>[2x]QTLLDALNVRVVGSGERVLVLAHGFGTDQSAWNRILPFFLRDYRVVLYDLVCAGSVNPDFFDFRRYTTLDPYVDDLLHILDALGIDQCAYVGHSVSAMIGILASIRRPELFSKLILIGASPRFLNDEDYHGGFEQGEIEKVFSAMEANYEAWVNGFAPLA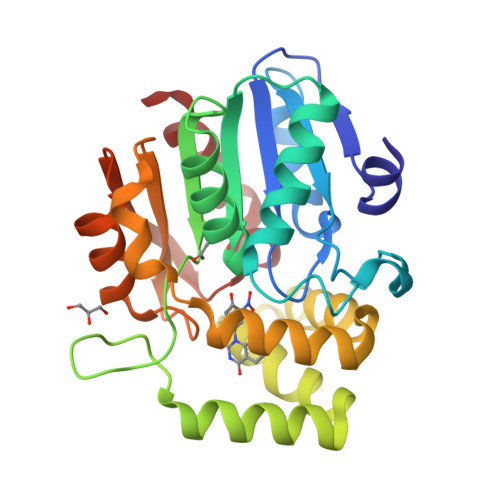VGADVPAAVREFSRTLFNMRPDITLFVSRTVFNSDMRGVLGLVKVPCHIFQTARDHSVPASVATYLKNHLGGKNTVHWLNIEGHLPHLSAPTLLAQELRRALSH> DLYFNPRFLADDPQAVADLSRFENGQELPPGTYRVDIYLNNGYMATRDVT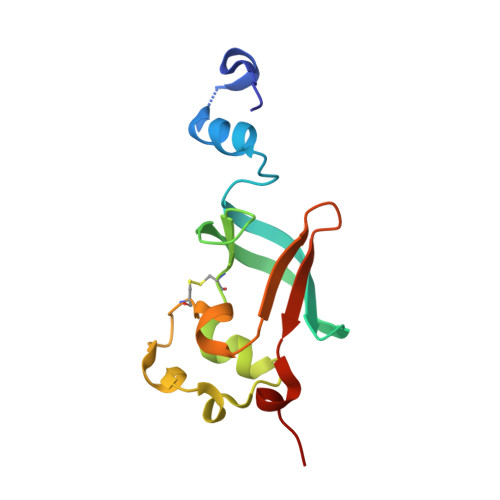FNTGDSEQGIVPCLTRAQLASMGLNTASVAGMNLLADDACVPLTTMVQDATAHLDVGQQRLNLTIPQAFMSNRAR({(2S)-3-(2-amino-6-oxo-1,6-dihydro-9H-purin-9-yl)-2-[(2S)-2-hydroxy-2-phosphonoethoxy]propoxy}methyl)phosphonic 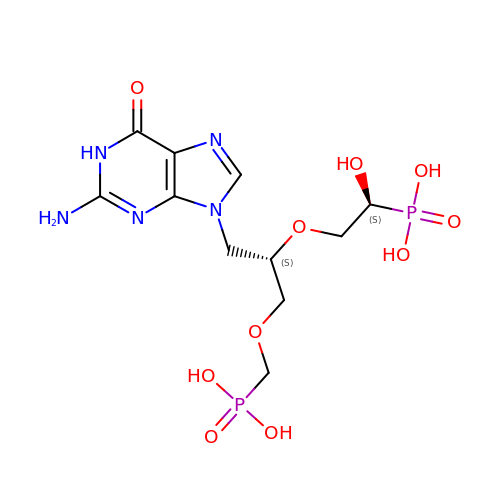acid | C11 H19 N5 O10 P2 | BCERVIXRVPEQOK-BQBZGAKWSA-N Here, we combine structural, cellular, and evolutionary analyses to demonstrate that SepF is the FtsZ anchor in the human-associated archaeon Methanobrevibacter smithii. M. smithii SepF binds to membranes and to FtsZ, inducing filament bundling. High-resolution crystal structures of archaeal SepF alone and in complex with the FtsZ C-terminal domain (FtsZCTD) reveal that SepF forms a dimer with a homodimerization interface driving a binding mode that is different from that previously reported in bacteria.

To further characterize the interaction between SepF and FtsZ, we crystallized MsSepFcore in complex with the FtsZCTD peptide and determined the structure of the complex at 2.7 Å resolution. The bound peptide is well-defined in the electron density for 10 out of 13 residues and adopts an extended conformation within a pronounced groove of the SepF monomer. The association is mediated by both hydrophobic and electrostatic interactions, the latter including 3 intermolecular ion pairs (FtsZ Asp 370 – SepF Arg 130, Asp 371 – Lys 115 and Asp 374 – Arg 118) and seven additional hydrogen bonds. Three of these H bonds are made by backbone atoms of the FtsZCTD peptide with the strand β3, partially extending the β-sheet. The archaeal-specific η1 insertion (residues 97-102) promotes the formation of a wider binding pocket compared to bacterial SepF and is involved in a network of hydrogen bonding interactions that contributes to stabilize the FtsZ-SepF complex. Furthermore, despite their evolutionary distance and sequence divergence, the structures of bacterial and archaeal SepF-FtsZ complexes share a partially conserved mode of interaction for the N-terminal part of the FtsZCTD (residues LDDFI in MsSepF and DLDV in CgSepF), which binds to a similar groove formed between α2 and β3 in the SepF monomer. However, the binding modes of the C-terminal half of FtsZCTD are markedly different between Archaea and Bacteria. In fact, in C. glutamicum this region interacts with residues from the two monomers of the SepF functional dimer at the α-helical interface, while in M. smithii it largely binds to only one monomer of the functional dimer, enlarging the monomer-peptide interface surface (600 Å2) with respect to that observed in C. glutamicum (390 Å2). In M. smithii, only the terminal residue of FtsZCTD (Phe377) binds to a surface hydrophobic pocket in the second SepF monomer at the β-sheet dimer interface. But a notable difference is the wider and deeper binding cleft of the FtsZ binding pocket in MsSepF formed between α2 and β3 through the archaeal-specific conserved η1 insertion. This results in a more important interaction of the FtsZCTD with the SepF monomer in Archaea than in Bacteria and could point towards an ancestral binding mode where a single monomer of SepF might have been sufficient for FtsZ binding.

> DDVSISPEQSFYEIMLIRPKTIDDINYVVDQVLEESNPVILDLSFLEKESPANFKLAGEKIKQMRSNYGAEALLLSRCNDKNLIIIAPKGVSLVRK;> QLDDFIDGIF As a model biocatalyst class, we selected carbamoylases, which promote the hydrolytic cleavage of N‐carbamoyl‐amino acids. Together with hydantoinases, they make up a scalable and widely‐employed enzymatic cascade for the production of enantiopure (un)natural amino acids (=hydantoin process). Based on its reportedly moderate activity for N‐carbamoylated‐ l ‐tyrosine, we produced and purified SmLcar, a carbamoylase from Sinorhizobium meliloti strain CECT 4114. Using this artificial link between enzyme activity and bacterial proliferation, we evolved the carbamoylase SmLcar to accept carbamoylated m‐substituted tyrosine analogs.

To rationalize the massive performance improvements of our engineered carbamoylases, we obtained crystal structures for SmLcar and the double mutant SmLcar_GC. Guided by the electron densities of unknown small molecules bound to the active sites of SmLcar and SmLcar_GC, we performed docking studies (YASARA) with the synthetic precursor, cam‐3iY, for both enzymes. Comparing the resulting structures of the wild‐type and the evolved variant revealed a striking difference in the orientation of the substrate in their respective binding pockets. Specifically, the critical Leu217Gly substitution identified in the first round enlarges the binding pocket and allows the aromatic side chain to flip by ≈90°. While our kinetic characterization reveals that this does not drastically alter the affinity of the ncAA precursor for the enzyme, as judged by the small differences in K M, this conformation appears to be highly beneficial for the attack of water at the adjacent metal‐binding site. Lastly, position 329 is distal to Gly217 and the introduced cysteine in SmLcar_GC (or Tyr in SmLcar_GY) interacts with the substrate to likely further lock it in an active conformation. The Leu217Gly substitution again proved crucial and boosted the turnover frequency (=0.23±0.01 s−1) and catalytic efficiency (89.9±13.2 M−1 s−1) by more than three and four orders of magnitude, respectively. Unexpectedly, the Phe329Cys substitution resulted in significantly improved reactivity, as SmLcar_GC fully converted cam‐3iY under these conditions. In stark contrast, installing a cysteine at position 329 proved highly beneficial, boosting the turnover number (4.84±0.39 s−1) and the catalytic efficiency (849±127 M−1 s−1) by another order of magnitude. When compared to the parent carbamoylase, SmLcar_GC displays a ≈70 000 times higher k cat and a ≈170 000‐fold improvement of k cat/K M. Combined, these results attest that our strategy of linking unrelated enzymatic activities to bacterial proliferation presents an effective means to engineer weakly active biocatalysts that do not fulfill a metabolic role.

>[2x]MGSSHHHHHHGSGLVPRGSAGMAAPGENRRVNADRLWDSLMEMAKIGPGVAGGNNRQTLTDADGEGRRLFQSWCEEAGLSMGVDKMGTMFLTRPGTDPDALPVHIGSHLDTQPTGGKFDGVLGVLSGLEAVRTMNDLGIKTKHPIVVTNWTNEEGARFAPAMLASGVFAGVHTLEYAYARKDPEGKSFGDELKRIGWLGDEEVGARKMHAYFEYHIEQGPILEAENKQIGVVTHCQGGWWLEFTLTGREAHTGSTPMDMRVNAGLAMARILEMVQTVAMENQPGAVGGVGQMFFSPNSRNVLPGKVVFTVDIRSPDQAKLDGMRARIEAEAPKICERLGVGCSIEAVGHCDPVTFDPKLVETVRGAAEKLGYSHMNLVSGAGHDACWAAKVAPTTMIMCPCVGGLSHNEAEDISREWAAAGADVLFHAVLETAEIVE>[2x]MGMLEARELLCERDERTLFSGLSFTLNAGEWVQITGSNGAGKTTLLRLLTGLSRPDAGEVLWQGQPLHQVRDSYHQNLLWIGHQPGIKTRLTALENLHFYHRDGDTAQCLEALAQAGLAGFEDIPVNQLSAGQQRRVALARLWLTRATLWILDEPFTAIDVNGVDRLTQRMAQHTEQGGIVILTTHQPLNVAESKIRRISLT;>MMFWRIFRLELRVAFRHSAEIANPLWFFLIVITLFPLSIGPEPQLLARIAPGIIWVAALLSSLLALERLFRDDLQDGSLEQLMLLPLPLPAVVLAKVMAHWMVTGLPLLILSPLVAMLLGMDVYGWQVMALTLLLGTPTLGFLGAPGVALTVGLKRGGVLLSILVLPLTIPLLIFATAAMDAASMHLPVDGYLAILGAL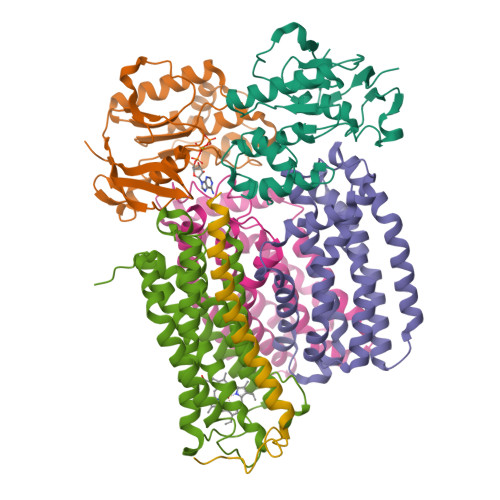LAGTATLSPFATAAALRISIQ[2x];> MWKTLHQLAIPPRLYQICGWFIPWLAIASVVVLTVGWIWGFGFAPADYQQGNSYRIIYLHVPAAIWSMGIYASMAVAAFIGLVWQMKMANLAVAAMAPIGAVFTFIALVTGSAWGKPMWGTWWVWDARLTSELVLLFLYVGVIALWHAFDDRRLAGRAAGILVLIGVVNLPIIHYSVEWWNTLHQGSTRMQQSIDPAMRSPLRWSIFGFLLLSATLTLMRMRNLILLMEKRRPWVSELILKRGRK;> MTPAFASWNEFFAMGGYAFFVWLAVVMTVIPLVVLVVHSVMQHRAILRGVAQQRAREARLRAAQQQEAA(2~{S},4~{R})-~{N}1-(1-aminocarbonylindol-3-yl)-4-fluoranyl-~{N}2-[3-(trifluoromethyloxy)phenyl]pyrrolidine-1,2-dicarboxamide | 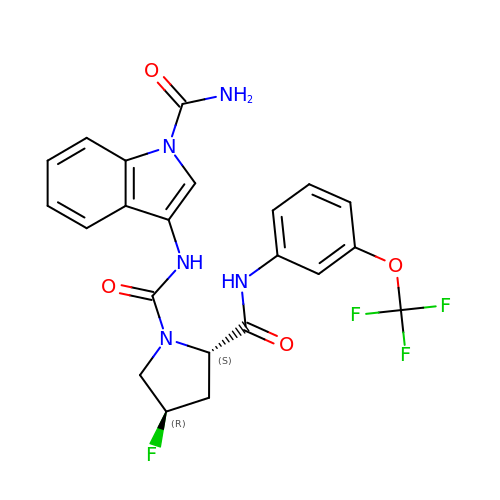C22 H19 F4 N5 O4 | PFNAXJGGZUYQGP-XIKOKIGWSA-N> MAPTWFYNTTNSEKLRELQHVLGGSAKLGYLTAKVTEILDVDLETVIRAKAIAAYRAVRVPVIVEHGALCIDALNGLPGALVKPFWESLDTRLCEVIPAGQRTARARGALCYCDGRERHVLIEETEGEIAPSARGTGGFHWDPIFIPKGQTRTFAEMSLDEKLS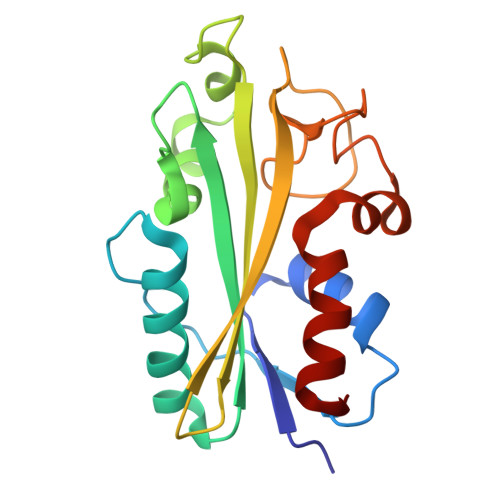FSPLGRLHTRLRTELGL> MGSSHHHHHHSQDPKPRCAATKANDHNQAAFGRQWQGRGIYKGRDSWSNIMLKEGDIVYGGAPGQSGFYFNKATLDAAGGSRAKLWESLQVLPHEKFGYRSKIQAYRVKRETIAGTGKAISQDPTRFGEGGGTQFFLSNYKTVLEPIDKPFEIGL;> MMQLDTYD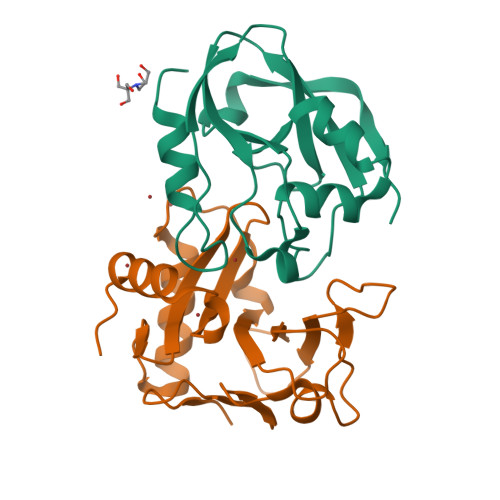GTLELAGITLGTATTREMLIKGSRLWEGWPEKSDGRTTSYRTIISTKKEKAGDIYIIADFSGAFITDAVLCSWRFAPEKLMMGIQKKVEGAITKNLRTWFYEKTHIQLPVSGSWGHIDAAYDPHNLTGTIVCNYRSAFHTEDEWRKYCKRNNIIY> VAAEDVVWRWSCDNGKCVKLKNDPRSSEPALSLEACKMFCNEYGLLWPRPTGEADLGNFLSKINLNSIEVKILKKGATDDLMEAAAKRFKEQVSLAIPRGSTPKLTGKAVDVYLVNENPNEKAFSLEMDESYGLRVSPSGADRVNATITANSFFGMRHGLETLSQLFVFDDIRDHLLMVRDVNISDKPVYPYRGILLDTARNYYS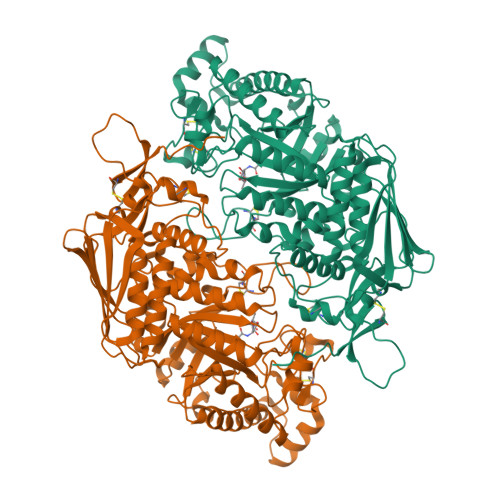IESIKRTIEAMAAVKLNTFHWHITDSQSFPFVTTKRPNLYKFGALSPQKVYTKAAIREVVRFGLERGVRVLPEFDAPAHVGEGWQDTDLTVCFKAEPWKSYCGEPPCGQLNPTKDELYQYLEDIYSDMAEVFDTTDIFHMGGDEVSEACWNSSDSIQNFMMQNRWDLDKESFLKLWNYFQQKAQDKAYKAFGKKLPLILWTSTLTNYKHIDDYLNKDDYIIQVWTTGVDPQIKGLLEKGYRLIMSNYDALYFDCGYGAWVGAGNNWCSPYIGWQKVYDNSPAVIALEHRDQVLGGEAALWSEQSDTSTLDGRLWPRAAALAERLWAEPATSWQDAEYRMLHIRERLVRMGIQAESLQPEWCYQNEGYCYS>[3x]GPGSSSKAISDISFQVERLAGQLSAF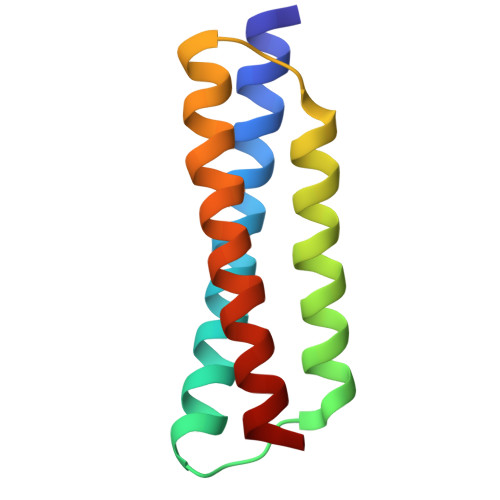DTVIGKGGKVEEKNLENLMEMLMNQLVKLDAISGDGDVKLKKKMQEERLHKYVEALDLLKIKNS>[6x]MTTDETTTTDATTITDATTIADATTRNAPKLPSPELYVEVTQFYARQMHRMDGDDF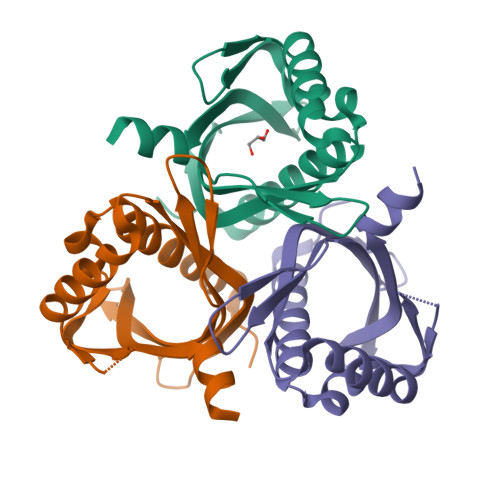GGFAATFVAGAEFRLAGGTVLTGPEAIEAGARAAAGRFDGAQPRHWFDMMTVEEADDGTVSTSYYATVTVTSAQGAVLVEPTCFVRDTLVRVSGVLRSRSRVIERDDLVVRARTQG> SLFKDDIQLNEHQVAWYSKDWTAVQSAADSFKEKAENEFFE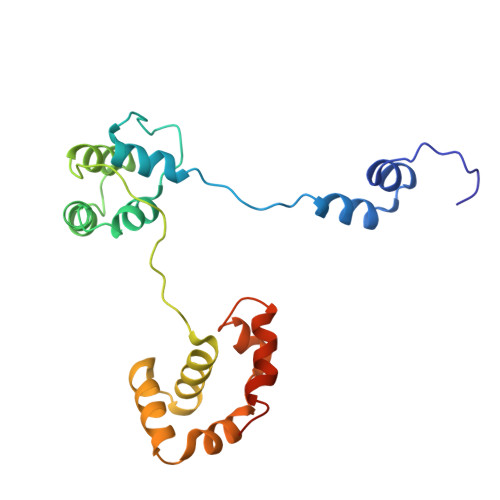IIGAINNKTKCSIAQKDYSKFMVENALSQFPECMPAVYAMNLIGSGLSDEAHFNYLMAAVPRGKRYGKWAKLVEDSTEVLIIKLLAKRYQVNTNDAINYKSILTKNGKLPLVLKELKGLVTDDFLKEVTKNVKEQKQLKKLALEWGLEHHHHHH> MHHHHHHTTPGEDHAGSF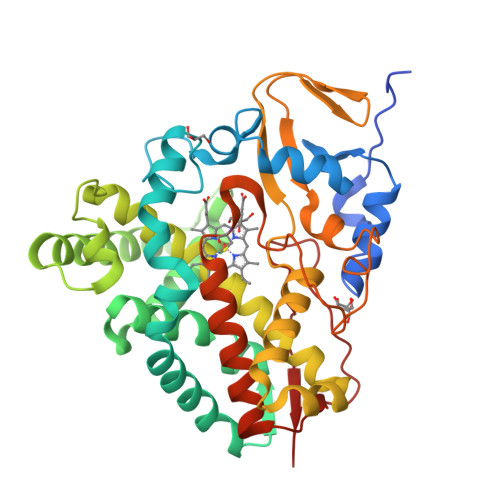YLPRLEYSTLPMAVDRGVGWKTLRDAGPVVFMNGWYYLTRREDVLAALRNPKVFSSRKALQPPGNPLPVVPLAFDPPEHTRYRRILQPYFSPAALSKALPSLRRHTVAMIDAIAGRGECEAMADLANLFPFQLFLVLYGLPLEDRDRLIGWKDAVIAMSDRPHPTEADVAAARELLEYLTAMVAERRRNPGPDVLSQVQIGEDPLSEIEVLGLSHLLILAGLDTVTAAVGFSLLELARRPQLRAMLRDNPKQIRVFIEEIVRLEPSAPVAPRVTTEPVTVGGMTLPAGSPVRLCMAAVNRDGSDAMSTDELVMDGKVHRHWGFGGGPHRCLGSHLARLELTLLVGEWLNQIPDFELAPDYAPEIRFPSKSFALKNLPLRWS> SKETKPLPDYVAWKDADALIVHSDKTLETKRSEFGTSIITPEEKLYIRNNVNTPPESILADRDGWKVEISGVKEPRTLTVAELKTLGLVTAATVLQCSGNGRKYFKDQLTGDQKMSGTPWTVGAAGCVIWSGVPLKAVVDALGGPAEGARFITGTGGEELPAGLDPKLLVVERSVPISNLDNVILAWEMNGRPLSLAHGGPLRMVVPGYSGVNNIKYVKAVAM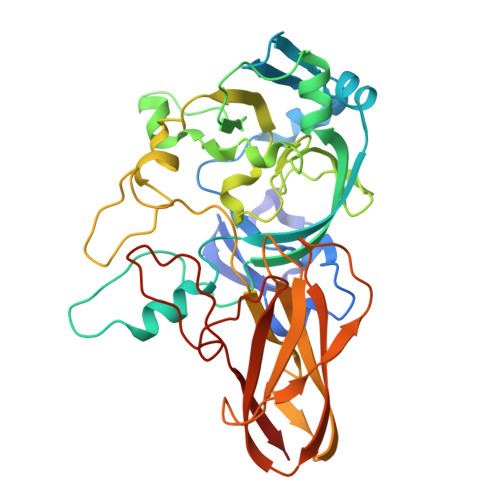TEVETDAKIQKTSYRVHALGEKGSPDQPSVWEQPVKSWITTPHEAAKAGQVQIAGVAFGGMNACKSVEVSVDGGQTWQEAEFIGPDLGRFAWRVFALSADLARGTYTLVSRATDTEGNVQPEETEMNGAGYGHNGWRAPAVKLTVA3-{[(4-methylphenyl)sulfonyl]amino}propyl pyridin-4-ylcarbamate | C16 H19 N3 O4 S | 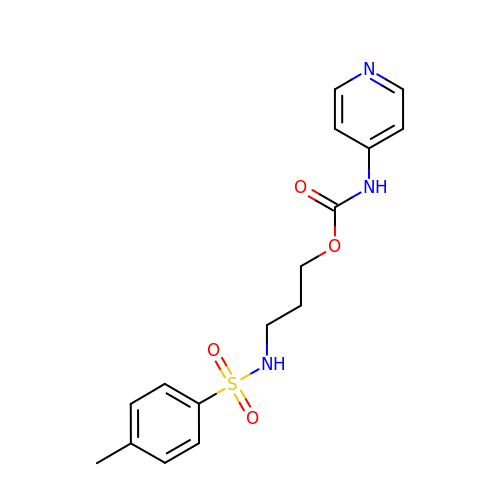ITYCDQJBLCTIID-UHFFFAOYSA-N> GPVEESVDRAVARVADTISSRPTNSESIPALTAAETGHTSQVVPSDTMQTRHVKNYHSRSESSIENFLCRSACVYYATYTNNSKKGFAEWVINTRQVAQLRRKLELFTYLRFDLELTFVITSAQQPSTASSVDAPVQTHQIMYVPPGGPVPTKVKDYAWQTSTNPSVFWTEGNAPPRMSIPFISIGNAYSCFYDGWTQFSRNGVYGINTLNNMGTLYMRHVNEAGQGPIKSTVRIYFKPKHVKAWVPRPPRLCQYEKQKNVNFSPIGVTTSRTDIITT;> SPSAEECGYSDRVRSITLGNSTITTQECANVVVGYGVWPEYLKDNEATAEDQPTQPDVATCRFYTLESVQWMKNSAGWWWKLPDALSQMGLFGQNMQYHYLGRTGYTIHVQCNASKFHQGCLLVVCVPEAEMGCSNLNNTPEFSELSGGDSARMFTDTQVGESNAKKVQTAVWNAGMGVGVGNLTIFPHQWINLRTNNSATLVMPYINSVPMDNMFRHNNLTLMIIPFVPLNYSEGSSPYVPITVTIAPMCAEYNGLRLASNQ;> GLPVMTTPGSTQFLTSDDFQSPSAMPQF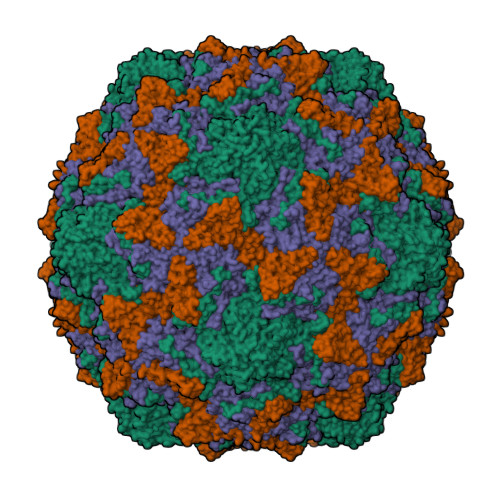DVTPEMQIPGRVNNLMEIAEVDSVVPVNNTEDNVSSLKAYQIPVQSNSDNGKQVFGFPLQPGANNVLNRTLLGEILNYYTHWSGSIKLTFMFCGSAMATGKFLLAYSPPGAGVPKNRKDAMLGTHVIWDVGLQSSCVLCVPWISQTHYRYVVEDEYTAAGYVTCWYQTNIVVPADVQSSCDILCFVSACNDFSVRMLKDTPFIRQDTFYQ;> MGAQVSTQKTGAHETGLNASGNSVIHYTNINYYKDAASNSANRQDFTQDPGKFTEPVKDIMVKTMPALN Compared to the RdRPs of other Flaviviridae representatives such as the NS5 of the Japanese encephalitis virus (JEV) and dengue virus (DENV) in the Flavivirus genus and the NS5B of the hepatitis C virus (HCV) of the Hepacivirus genus, the pestivirus NS5B contains a unique ∼90-residue N-terminal domain (NTD) that does not have notable sequence homology to any other viral or host proteins. The global conformation of our CSFV NS5B structures is consistent with the recently reported CSFV structure with an RMSD value of 0.9 Å (95% coverage) between the reported structure and our representative C-682 structure. These structures together reveal that the NTD adopts a globular α/β fold with an α-β-α-β-β-α pattern. The NTD interacts with the palm of the RdRP core intra-molecularly with a mixture of hydrophobic and hydrogen bonding interactions. Collectively, these biochemical data indicated that the RNA synthesis fidelity of CSFV NS5B is fine-tuned by its NTD through the intra-molecular interactions with the RdRP palm.

To better understand the nature of the NTD–RdRP intra-molecular interface interactions and whether they regulate the RdRP fidelity, we designed point mutations at the Y471 and E472 sites in the context of the WT NS5B and the N- and C-terminal deletion mutants. Crystallization screenings were performed for all the NTD containing mutant constructs and four of them were successfully crystallized with one construct crystallized under two different conditions. Among these five structures, three of them (Y471A and two forms of C-672_Y471A) maintain the WT conformation with the NTD–RdRP intra-molecular interface maintained. The NTD–RdRP intra-molecular interactions are fully disrupted, and the NTD is rather involved in a non-intensive three-way interaction involving two symmetry-related neighboring NS5B molecules in the crystal lattice. These structural data together suggest that the selection of Y471-E472 mutation sites is valid in perturbing the NTD–RdRP interface, but the interface may not necessarily be fully disrupted by some of the mutations. The effect of E472A mutation was highly consistent with AA mutation (compare lanes 4/8/14/18 to 5/9/15/19), while the effect of Y471A mutation was slightly smaller than that of the E472A and AA mutations (compare lanes 3/7/13/17 to 4/8/14/18 and 5/9/15/19). Although NTD–RdRP disengagement, a situation mimicked by the crystallographic open conformation state in a crystal lattice or the N-91 construct in solution, results in fidelity reduction, engaged NTD–RdRP with perturbation from point mutations can achieve similar level of fidelity reduction.

> MSNWVMQEENKQGNLTPLFEELLQQCPPGGQNKTAHMVSAYQLAQGNWMPTSCHVFMGTISARRTKTHPYEAYVKLRELVEEHKMKTLCPGSSLGKHNDWIIGKIKYQGNLRTKHMLNPGKVAEQLCREGHRHNVYNKTIGSVMTATGIRLEKLPVVRAQTDTTNFHQAIRDKIDKEENLQTPGLHKKLMEVFNALKRPELESSYDAVEWEELERGINRKGAAGFFERKNIGEILDSEKNKVEEIIDNLKKGRNIKYYETAIPKNEKRDVNDDWTAGDFVDEKKPRVIQYPEAKTRLAITKVMYKWVKQKPVVIPGYEGKTPLFQIFDKVKKEWDQFQNPVAVSFDTKAWDTQVTTKDLELIKDIQKYYFKKKWHKFIDTLTMHMTEVPVICADGEVYIRKGQRGSGQPDTSAGNSMLNVLTMVYAFCEATGVPYKSFDRVAKIHVCGDDGFLITERALGEKFASKGVQILAEAGKPQKITEGDKMKVAYQFDDIEFCSHTPIQVRWSDNTSSYMPGRNTTTILAKMATRLDSSGERGTIAYEKAVAFSFLLMYSWNPLIRRICLLVLSTELQVKPGKSTTYYYEGDPISAYKEVIGHNLFDLKRTSFEKLAKLNLSMSVLGAWTRHTSKRLLQDCVNMGVKEGNWLVNADRLVSSKTGNRYIPGEGHTLQGRGSSSHHHHHH> MGSSLRPLYMD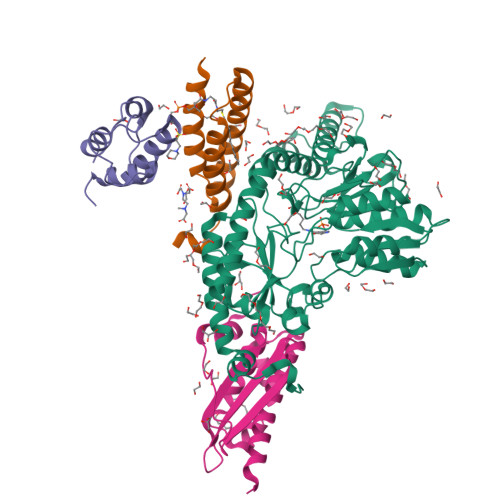VQATTPLDPRVLDAMLPYLINYYGNPHSRTHAYGWESEAAMERARQQVASLIGADPREIIFTSGATESNNIAIKGVARFYRSRKKHLITTQTEHKCVLDSCRSLEAEGFQVTYLPVQKSGIIDLKELEAAIQPDTSLVSVMTVNNEIGVKQPIAEIGRICSSRKVYFHTDAAQAVGKIPLDVNDMKIDLMSISGHKIYGPKGVGAIYIRRRPRVRVEALQSGGGQERGMRSGTVPTPLVVGLGAACEVAQQEMEYDHKRISKLSERLIQNIMKSLPDVVMNGDPKHHYPGCINLSFAYVEGESLLMALKDVALSSGSACTSASLEPSYVLRAIGTDEDLAHSSIRFGIGRFTTEEEVDYTVEKCIQHVKRLREMSPLWEMVQDGIDLKSIKWTQH;> MAASSRAQVLALYRAMLRESKRFSAYNYRTYAVRRIRDAFRENKNVKDPVEIQTLVNKAKRDLGVIRRQVHIGQLYSTDKLIIENRDMPRT;> STIEERVKKIIGEQLGVKQEEVTNNASFVEDLGADSLDTVELVMALEEEFDTEIPDEEAEKITTVQAAIDYINGHQA;> MALSTQVVDHYENPRNVGSLDKTSKNVGTGLVGAPACGDVMKLQIQVDEKGKIVDARFKTFGCGSAIASSSLATEWVKGKTVEEALTIKNTDIAKELCLPPVKLHCSMLAEDAIKAALADYKLKQEPKKGEAEKKLEHHHHHH>[2x]MAHHHHHHMTNNRVRVAVTGAAGQIGYALVFRIASGQMFGPNTEVELNLLELEPALPSLEGVAMELDDCAFPLLKRIVCTADLNKAMDGVNWALLVGSVPRKQGMERSDLLQINGGIFTKQGQAINDYASDDVRVFVVGNPCNTNCLIAMNHAKDVPSDRFYAMTTLDELRARTQLAKKAGVDITAVTQMTIWGNHSATQYPDFYNAKINGTS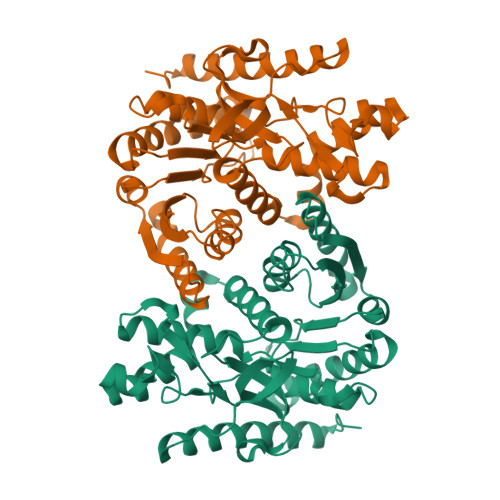AAQVINDETWLKETFVSTVQQRGAAVIKARGSSSAASAANAIITGVNHLVTDTPAGESFSMCRRSKGEYGVDEGLIFSFPCRREHGELKVVENLEFNDFGRERFNTTLNELRSERDTVKSLGLLD The protein N is a multifunctional protein that packs the genomic RNA and enhances the efficiency of virus transcription and assembly. N contains an N-terminal domain, involved in RNA binding, and a C-terminal (NCTD) involved in RNA binding, protein dimerization, and interaction with the viral membrane protein (M). The SARS-CoV-2 NCTD folds into a helical core with a protruding β-hairpin employed for protein dimerization. Here we report the crystal structure of the C-terminal domain (NCTD) in open and closed conformations and in complex with guanine triphosphate, GTP.

The structure of the binary complex NCTD-GTP was solved in two different space groups, P21 and P1, to a resolution of 1.8 and 2 Å, respectively. Both crystal forms contain two protein dimers in the asymmetric unit. However, in the space group P21 there is one molecule of GTP bound to one of the dimers, whereas in the P1 the asymmetric unit contains two molecules of GTP, each bound to one dimer. The electron density map is well defined for the three GTP molecules, which present temperature factors that increase from the guanine moiety to the phosphates, suggesting that the guanine is well anchored to the protein and the phosphates are more flexible. In the two crystal forms the GTP binds to a cleft between the two subunits of the dimer, and adjacent to the β-hairpin in the closed conformation. One side of the guanine ring establishes a π–π T-shaped interaction (edge-to-face) with the indole ring of W330 and hydrophobic interactions with K338. The other side of the guanine ring stacks over the guanidinium group of R259, which makes hydrogen bonds with the OH– groups of the ribose ring. At the bottom of the cleft the guanine moiety interacts with the M317 and with the main chain of the residues K338 and A336. These interactions suggest high specificity for guanine, as other nitrogen bases have not as many favorable interactions as the guanine. Importantly, the C-terminal tail of the symmetry-related dimer also contributes to the GTP binding, covering the cleft as a lid, with Van der Waals and hydrophobic interactions between T362´ and the ribose and with the π–π stacking between P364´ and W330.

>[4x]MGSSHHHHHHGENLYFQSTKKSAAEASKKPRQKRTATKAYNVTQAFGRRGPEQTQGNFGDQELIRQGTDYKHWPQIAQFAPSASAFFGMSRIGMEVTPSGTWLTYTGAIKLDDKDPNFKDQVILLNKHIDAYKTFP> YQTERFTKFSDTLKEFKIEQNNEQNPIDPFNIIREFRSAAGQLALDLANSGDESNVISSKDWELEARFWHLVELLLVFRNADLDLDEMELHPYNSRG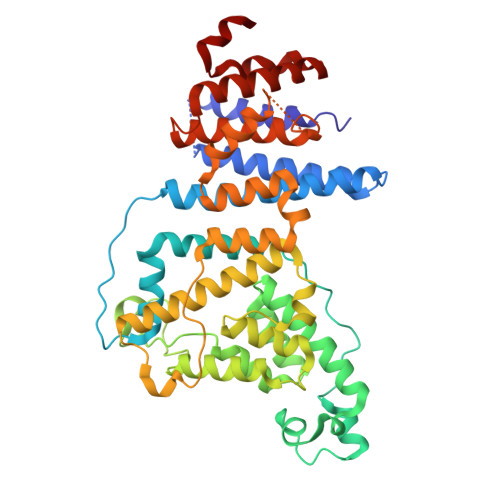LFEKKLMQDNKQLYQIWIVMVWLKENTYVMERPKNVPTSKWLNSITSGGLKSCDLDFPLRENTNVLDVKDKEEDHIFFKYIYELILAGAIDEALEEAKLSDNISICMILCGIQEYLNPVIDTQIANEFNTQQGIKKHSLWRRTVYSLSQQAGLDPYERAIYSYLSGAIPNQEVLQYSDWESDLHIHLNQILQTEIENYLLENNQVGTDELILPLPSHALTVQEVLNRVASRHPSESEHPIRVLMASVILDSLPSVIHSSVEMLLDVVKGTEASNDIIDKPYLLRIVTHLAICLDIINPGSVEEVDKSKLITTYISLLKLQGLYENIPIYATFLNESDCL>[2x]AHHHHHHGSRELVEIIKGIGIEGAKEVEEKVDRQFYALQYLFRHQDPEMFIKLVIANSLVSYQLTG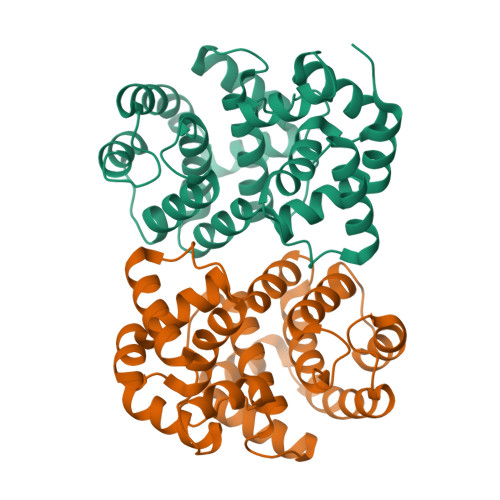RGEDWWWEFARYFSGREVDSIWKAYGEFLPKSKNNRRLIEAKLNRIRKVEGFLSTLTLKDLEGYYKNMKMLWKALIKIMGSREDSKTIVFTVKMFGYASRIAFSRFIPYPMEIPIPEDLRIKSVTSKLTQEKPTKFWMKIGQESGVPPLHIDSLIWPLLGNADLTPLDIELRNKLMKLTELLGL>MEFSSFLFTILLFSLNISPLVSAHGSNHEDFLKCLSYRMNDNTVEPKVIHTSKDSSFFSILDSSIQNPRFSVSETPKPVSIITPVKASDVQTVIRCAQLHGIHVRTRSAGHCYEGLSYIAYN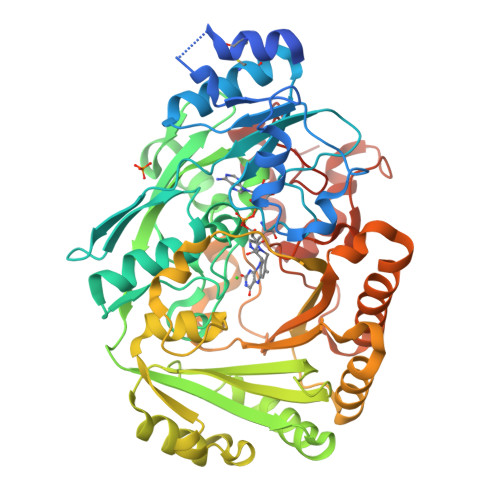KPFAVIDLRNLRSISLDVDNRTGWVQTGATAGELYYEIGKTTKSLAFPAGIHPTVGVGGQFSGGGYGTLLRKYGLAADNIIDALVVDASGRILDRQAMGEDYFWAIRGGGGSSFGVILSWKVKLVDVPSTITVFKVQKTSKKEAVRIIKKWQYAADKVPDDLFIRTTLERSNKNAVHALFTGLYIGPVNNLLALMEEKFPELGLEKEGCEEMSWIESVLWFADFPKGESLGVLTNRERTSLSFKGKDDFVQEPIPEAAIQEIWRRLEAPEARLGKIILTPFGGKMSEMAEYETPFPHRGGNLYEIQYVAYWREEEDKNKTETDKYLKWVDSVYEFMTPYVSKSPRGAYVNFKDMDLGMYLGKKKTKYEEGKSWGVKYFKNNFERLVRVKTRVDPTDFFCDEQSIPLVNKVT[2x]>[2x]MALQFTLNQDAPASAAVDCIVVGAFADKTLSPAAQALDSASQGRLTALLARGDVAGKTGSTTLLHDLPGVAAPRVLVVGLGDAGKFGVAPYLKAIGDATRALKTGAVGTALLTLTELTVKARDAAWNIRQAVTVSDHAAYRYTATLGKKKVDETGLTTLAIAGDDARALAVGVATAEGVEFARELGNLPPNYCTPAYLADTAAAFAGKFPGAEAEILDEAQMEALGMGSLLSVARGSANRPRLIVLKWNG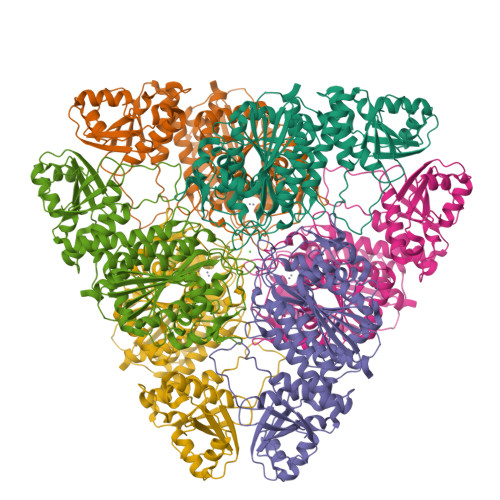GGDARPYVLVGKGITFDTGGVNLKTQGGIEEMKYDMCGGATVIGTFVATVKAELPINLVVVVPAVENAIDGNAYRPSDVITSMSGKTIEVGNTDAEGRLILCDALTYAERFNPEALVDVATLTGACMVALGHQTAGLMSKHDDLANELLAAGEHVFDRAWRLPLWDEYQGLLDSTFADVYNIGGRWGGAITAGCFLSRFTENQRWAHLDIAGVASDEGKRGMATGRPVGLLTQWLLDRAA>MVKVAYVQMNPQILEPDKNYSKAEKLIKEASKQGAQLVVLPELFDTGYNFETREEVFEIAQKIPEGETTTFLMDVARDTGVYIVAGTAEKDGDVLYNSAVVVGPRGFIGKYRKIHLFYREKFFFEPGDLGFRVFDLGFMKVGVMICFDWFFPESAR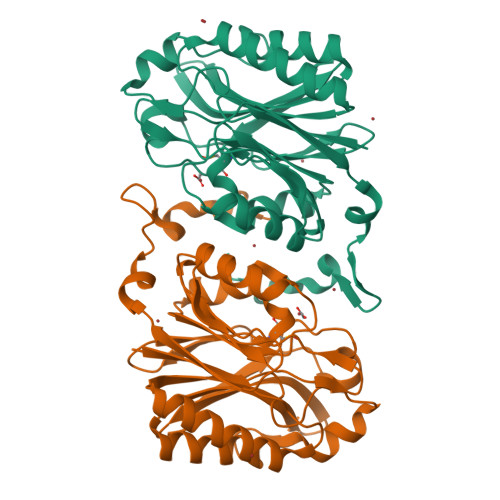TLALKGADVIAHPANLVMPYAPRAMPIRALENKVYTVTADRVGEERGLKFIGKSLIASPKAEVLSMASETEEEVGVAEIDLSLVRNKRINDLNDIFKDRREEYYFR[2x]> ETPPRFTRTPVDQTGVSGGVASFICQATGDPRPKIVWNKKGKKVSNQRFEVIEFDDGSGSVLRIQPLRTPRDEAIYECVASNNVGEISVSTRLTVLREDQIPRGFPTIDMGPQLKVVERTRTATMLCAASGNPDPEITWFKDFLPVDTSNNNGRIKQLRSESIGGTPIRGALQIEQSEESDQGKYECVATNSAGTRYSAPANLYVRELREVRRVPPRFSIPPTNHEIMPGGSVNITCVAVGSPMPYVKWMLGAEDLTPEDDMPIGRNVLELNDVRQSANYTCVAMSTLGVIEAIAQITVKALPKPPGTPVVTESTATSITLTWDSGNPEPVSYYIIQHKPKNSEEPYKEIDGIATTRYSVAGLSPYSDYEFRVVAVNNIGRGPASEPVLTQTSEQAPSSAPRDVQARMLSSTTILVQWKEPEEPNGQIQGYRVYYTMDPTQHVNNWMKHNVADSQITTIGNLVPQKTYSVKVLAFTSIGDGPLSSDIQVIT;> SERCDDWGLDTMRQIQVFEDEPARIKCPLFEHFLKYNYSTAHSSGLTLIWYWTRQDRDLEEPINFRLPENRISKEKDVLWFRPTLLNDTGNYTCMLRNTTYCSKVAFPLEVVQKDSCFNSAMRFPVHKMYIEHGIHKITCPNVDGYFPSSVKPSVTWYKGCTEIVDFHNVLPEGMNLSFFIPLVSNNGNYTCVVTYPENGRLFHLTRTVTVKVVGSPKDALPPQIYSPNDRVVYEKEPGEELVIPCKVYFSFIMDSHNEVWWTIDGKKPDDVTVDITINESVSYSSTEDETRTQILSIKKVTPEDLRRNYVCHARNTKGEAEQAAKVKQKVAAHHHHHH

Vertebrate type-IIa RPTPs comprise LAR, PTPσ and PTPδ, which share common domain architecture with a single transmembrane (TM) helix flanked by a large extracellular domain (ECD) and cytoplasmic tandem PTP domains: the membrane-proximal PTP domain (D1) is catalytically active, whereas the membrane-distal PTP domain (D2) is inactive. In mammals, presynaptic type-IIa RPTPs form trans-synaptic adhesion by specifically binding to their cognate postsynaptic organizers through their ECDs for inducing synaptic differentiation of neurons. To date, five different types of postsynaptic organizers for type-IIa RPTPs have been reported: interleukin-1 receptor (IL-1R) accessory protein (IL-1RAcP)7, IL-1RAcP-like-1 (IL1RAPL1)8, neurotrophin receptor tyrosine kinase C (TrkC), netrin-G ligand-3 (NGL-3)1011 and Slit- and Trk-like (Slitrk) family proteins. To elucidate the structural basis for decoding the ‘splice-insert signaling code' in the type-IIa RPTPs, we determined the crystal structures of PTPδ-ECD in complex with IL-1RAcP-ECD and IL1RAPL1-ECD.

To structurally explain these differences between IL1RAPL1 and IL-1RAcP, we also determined the crystal structure of IL-1RAcP-ECD in complex with PTPδ containing three Ig domains and two Fn domains (Ig1-Fn2) at 3.25 Å resolution. Similarly to the PTPδIL1RAPL1 complex, the Ig1-Fn2 domains of PTPδ bind to IL-1RAcP-ECD at a ratio of 1:1. The Ig1-Fn2 domains of PTPδ exhibit an elongated shape with a length of 160 Å along the longest axis. The Ig1–Ig3 domains of IL-1RAcP are arranged in an L-shape similar to those of IL1RAPL1, except that the relative orientation between the Ig1 and Ig2–Ig3 domains is changed by 20 degree. Correspondingly, the Ig3 domain of IL-1RAcP does not interact with PTPδ in contrast to that of IL1RAPL1. The interface between the IL-1RAcP Ig1 and PTPδ Ig2 domains comprises both hydrophobic and hydrophilic interactions with a buried surface area of 726 Å2. Although Arg196 of PTPδ is positioned in close proximity to Asp30 of IL-1RAcP, no observed electron density of its side chain guanidino group indicates that the interaction between Arg196 of PTPδ and Asp30 of IL-1RAcP is substantially weak. Basically, meA does not extensively interact with IL-1RAcP in the PTPδ Ig1-Fn2IL-1RAcP-ECD complex, consistent with the finding that the variation of meA does not affect the affinity for IL-1RAcP. The interface between the IL-1RAcP Ig1 and PTPδ Ig3 domains buries a surface area of 906 Å2. Therefore, the interface mediated by PTPδ Ig3 is more critically important for binding to IL-1RAcP than for binding to IL1RAPL1, consistent with the finding that PTPδ Ig3 is essential for binding to IL-1RAcP but not to IL1RAPL1.>[12x]MGLNFFRKAAPEVRTEPVAERKASVTGRIVAMASGAGRPVWGPRDTVSLMRTGFAGNPVGFRSVKLIAEATAAVPLICQDAERRYEIHPVLDLLRRPNAGQGRAELFEALIGQILLSGNGYLEAVCPEPGVPRELHVLRSDRMAVVPGADGWPVGYDYTVGGRKHRFDMTGHPDPICHIKSFHPTDDHYGLSPMQAAAVALDVHNAASAWSKALLDNAARPSGAIIYKGADGQGVLAPEQYERLIFEMETHHQGARNAGRPMLLEGGLDWKPMGFSPSDMEFHETKAAAAREIALAFGVPPMLIGIPGDATYANYAEANRAFYRLTVLPLLTRVSAALAWWLSGYLGAQIELKPDLDQVPALAVERDQLWARIGAAGFLSNSEKRVLLGLPPTAEG;>MMLNEVTAVPGTALPVAEFRDHLRLGTGFADLGAEDAALLSYLRAAIAAIEGRTAKALISRGFRLALTAWRWGDMQTLPIAPVATVTALRLVDAAGVETPVAAGWRLVPDMARPRIEALGAMLPMIPTGGRVEIDFTAGFGASWSALPVDLAQAVFLLAAQYYELRHDGAAEGGAMPFGVMALIERWRTVRVLGGRP[12x];>MSRPRLNRLLVLEEAVRVADGAGGHRLDWQAKGEVWAEVTAGSGSERAGEFVTLASVPFTIVVRAAPVGAARRPRPEQRFREGARIFRILAVAERDREGHYLSCFAREEVVA[6x];>MSYAVAGALQAAVYQQLRADAVLAALVGTAVYDAVPPGPLAGTYVSLGPEDVADASDKTGAGAVHDFVISVITDAAGFATAKAAAAAVSDALVGADLVLSRGRLVGLWFLRAKARRVEKADMRRIDLVFRARVEG[6x];>[30x]MAAQNGKDLLIKLDLTGSGQFETIAGLRATRISFNAETVDVTSLESQGGWRELLGGAGVRSASISGAGVFKDADTDERARQIFFDGEVPEFQVIIPDFGIVQGPFMITSIDYAGSHNGEASYELAMASAGALSFTAI;>[6x]MAFHEVRFPANLSFGSVGGPERRTEIVTLSSGHEERNSPWAHSRRHYDAGVGLRSLDDVERLIAFFEARGGQLHGFRWKDWADFKSCPASRAVA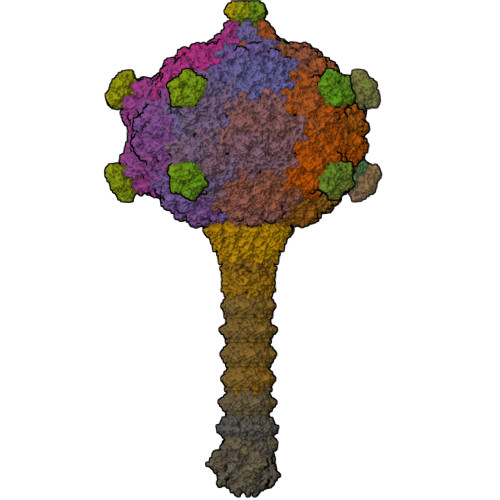HEDQLIGMGDGVTTAFQLVKTYVSGGQSYLRPIVKPVEGTVKLGIAGDHQAEAVNFAVDHATGIVSFNEPPPQGARVTAGFEFDVPVRFDTDRIAVSVQSFQAGDLPQVPVVEVRI;>[3x]MAYPESLKAHLQGGVTTLARAWALARADGRVLGFTDHDVVLRFDGISFEPGSGMTAKAVLQGTGLSVDNTESYGALSSEAITEADLLAGRYDGAAVTVWLVNWADPAMRAVIFRGHLGEVSRGAGAFTAELRGLTAALGQEQGRIYHPRCAAVLGDGRCRFDLTKDGYALEAALGGVDEAVVLRLAEGAGFEDRWFEKGRLVVLDGAAAGLIGVVKNDRLQADGSRLIELWQRLGANPVAGDRVRIEPGCDKRAGTCRLKFDNFLNFRGFPHIPGEDWMVSYPVQSGTNDGGSLFR;>[3x]MATILLSAAGAAIGGGFGGTVLGLSGAVIGRAVGATLGRVIDQRLLGSGSQSVETGRVDRLRLSSASEGEAVGRLWGRMRVAGQVIWATRFFESASVEKSGKGVPRATVTSYSYSLSLALALCEGEILRVGRVWADGSEIEVSGLNMRVYRGGEDQLPDPKIAAVEGAEAAPAYRGIAYVVLEDLQLAPFGNRVPQFTFEVVRAAQGALAEAEPDLTRGLRAVALIPGTGEYALATTPVYLATGSGVTATQGVANQNAPGGQTDLVAALERLDEELPNCGAVSLVVSWFGDDLRCGACDVKPKVASVAEEGANMPWRVAGLERAGAEEVPRLSGQSVYGGTPADAAVIEAIAALRAAGKAVTFYPFILMAQLAGNGLPDPWNPGSAQPALPWRGRITLSVAPGRAGSPDGTAAAEAQVAGFFGAASPGDSAIAGGEVVYSGPEEWSMRRFILHYAHLCQLAGGVDAFCIGTEMVALTQIRGPSNSFPAVAAFRQLAGEVKAILGPGCKIGYAADWSEYWGYAPGNGERFFHLDPLWADENIDFIGIDNYLPLSDWRDGADHADAGWGSIHALDYLRSNIEGGEYYDWFYAAPEHRAAQIRTPITDGDHDEPWIWRAKDLRNWWLNDHHERVGGLRSEVATAWVPQSKPIWFTEMGCAAIDKGTNQPNKFLDPKSSESGLPHHSDGRRDELIQMQYLRAMTGYWGEAARNPVSAVYGGPMLDMSRAHVWAWDARPWPQFPLNTALWSDGENYARGHWISGRAVAQPLASVVAEICGAAGITEIDVSGLYGLVRGYTMTGDQTGRAGLQALMLAYGFEALERDGQLVFRMRDGRVAADLAAADLALGEGEAVVETVRAAEAEIAGRVRLAYVEAEGDFEVKAVEAVFPDAAAGAAAGSELSLALTRAQAQGIVGRWLAEARVARDTARFALPPSRGHLGTGDVVRLDLPEGKRRYRIDRVEQAGLIQVEAVRVEPGIYAPADEVEDPASLRPFAAPVPVTAVFLDLPLMKGDEDPVAPHLAVTATPWPGTVAVWSSDEDAGYALNASLGTRAVIGQTLTPLFRARPGVWDRGAALRVRLASGALDSATAAKVLNGANAMAIGDGSSENWEVFQFAEAALVEGKIWDISLRLRGQLGTDALMPEVWPEGSVVVALNGAPEQILLPSAARGLARHYRIGAAVRSYDDPSFVHRIEAFAGAGLRPFSPCHLRAEPGASGWAFRWVRRTRIDGDSWQGYEVPLGETAELYLVRVLEGTAVKREVTVGEASWSYPAALQAADGIAGAFTLEVAQVSDVYGPGLAARITVGA;>[55x]MDVFAKHAVSLESPAVRHYEITPSDSTDLARRPRALRVQTGGTLVLRDETGITVTYTVFAGEILPVRPVRVLATGTTATAVGWE;>MPEGADPVAEVKTALAGFLKEVKGFQDDVKTRLQQQEERVTMLQTKTYAGRHALAAAATEEAPHQKAFAAYLRTGDDDGLRGLSLEGKALNSAVAAEGGYLVDPQTSETIRGVLRSTASLRQIASVVNVEATSFDVLVDKTDMGSGWASETAALSETATPQIDRITIPLHELAAMPKASQRLLDDSAFDIETWLANRIADKFARAEAAAFISGDGVDKPTGFLTKTKVANGAWAWGSLGYVATGAAGDFAAVNASDAVVDLVYALGAEYRANASFVMNSKTAGAVRKMKDADGRFLWADSLAAGEPARLMGYPVLIAEDMPDIAANAYAIAFGDFGNGYTIAERPDLRVLRDPFSAKPHVLFYASKRVGGDVSDFAAIKLLKFAA[145x];>MIALGLGLGLAANGGPALRRYAVNGVAPVAVLDFERHFLSHPLALTRATSATYADALRAVQTAPADTPRYDYSTGKRALLLEASATNLLPNSAQFEAASWGKTRASVLANAALAPNGTMTADKLVEDTSNNSHFVARTGTQIAAGTSVTASIFVKAAERRWFALVTADSANAFRTTYFDLQTGTLGVVSQGAAGHVAQIVAAGNGWYRCSVTQTQAASGNFNFYPSVASANGATSYPGDGASGLYLWGAQLEAGAAVSSVIPTEAAAVTRAADLASVAVAAGSYDLRRVDAAGTAVTKGVAHPGGALTIGAGSLYLLSLFPAGAL[10x]>MGEAAIEAVEEMERLLREASSILRVEPAKLPKTVERFFEEWKDQRKEIERLKSVIADLWADILMERAEEFDSMKVVAEVVDADMQALQKLAERLAEKGAVGCLMAKGEGKVFVVTFSGQKYDARELLREIGRVAKGSGGGRKDVAQGAVQQLLDREEMLDVIF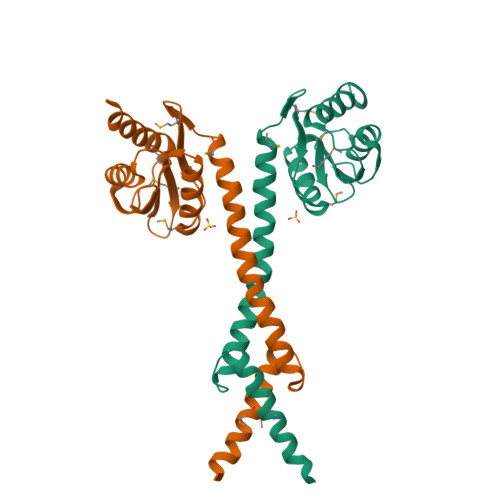RFLSEHEG[8x]tert-butyl 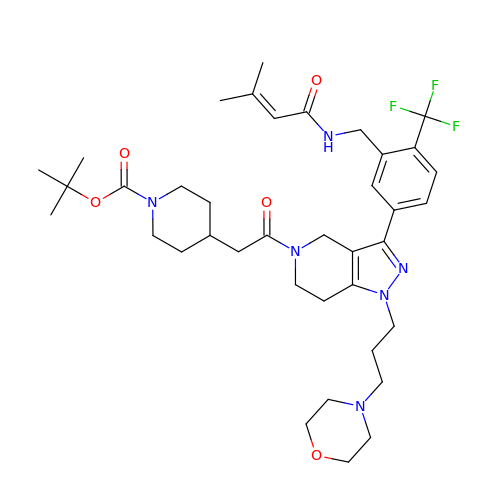4-(2-{3-[3-{[(3-methylbut-2-enoyl)amino]methyl}-4-(trifluoromethyl)phenyl]-1-[3-(morpholin-4-yl)propyl]-1,4,6,7-tetrahydro-5H-pyrazolo[4,3-c]pyridin-5-yl}-2-oxoethyl)piperidine-1-carboxylate | C38 H53 F3 N6 O5 | VGHVCBNZEGIXOJ-UHFFFAOYSA-N> XQLD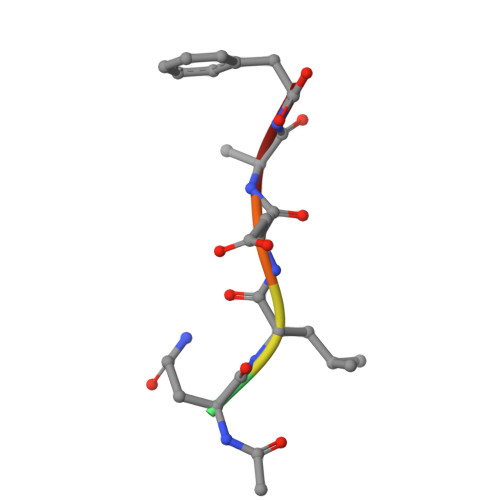AF>MGSSHHHHHHSQDPSQFIRRDIAQTVNGSLTLTQQTNLSAPLVSSSTGEFGGSLAANRTFTIRNTGAPTSIVFEKGPASGANPAQSMSIRVWGNQFGGGSDTTRSTVFEVGDDTSHHFYSQRNKDGNIAFNINGTVMPININASGLMNVNGTATFGRSVTANGEFISKSANAFRAINGDYGFFIRNDASNTYFLLTAAGDQTGGFNGLRPLLINNQSGQITIGEGLIIAKGVTINSGGLTVNSRIRSQGTKTSDLYTRAPTSDTVGFWSIDINDSATYNQFPGYFKMVEKTNEVTGLPYLERGEEVKSPGTLTQFGNTLDSLYQDWITYPTTPEARTTRWTRTWQKTKNSWSSFVQVFDGGNPPQPSDIGALPSDNATMGNLTIRDFLRIGNVRIVPDPVNKTVKFEWVE[12x]

The proximal half-fiber is formed by a parallel homo-trimer of gp34. The protein is a highly intertwined trimer containing a 2 nm-wide triple β-helix domain interspersed with three wider domains in which each of the monomers forms an anti-parallel β-sheet. The long tail fibers recognize the outer membrane protein C (OmpC) or the lipopolysaccharide (LPS) of E. coli and are responsible for the initial and reversible attachment of the virion. The carboxy-terminal parts of gp34 that we crystallized occupy the part of the proximal tail fiber closest to gp35 (the “knee”).

Crystals belonging to two different space groups (P21 and R32) were obtained for gp34(894–1289). The structure of the R32 crystal form was solved by molecular replacement, using the hexagonal setting H32. Four trimers (i.e., twelve identical protein chains) were found in the asymmetric unit. Here, manual fitting and refinement led to a final model consisting of 4736 residues (894–1288 of chain A, 894–1288 of chain B, 890–1287 of chain C, 893–1287 of chain D, 890–1287 of chain E, 893–1288 of chain F, 894–1288 of chain G, 894–1287 of chain H, 895–1288 of chain I, 895–1288 of chain J, 897–1287 of chain K, and 894–1288 of chain L). For final refinement at 3.0 Å resolution, secondary structure restraints were used as without them the model tended to get distorted.> GMGKGKSAIESQI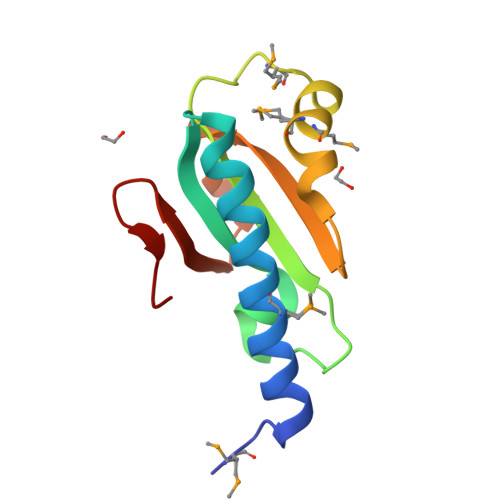RMLKLAKEIVEEVASSFPNLEEVYIFGSRARGDYLDTSDIDILFVFKGIKEMNVFDRMYMVSRFIRGNVDYIVLDEGEKDRVKDKVLFWKREKGFVLL>[6x]MADFKFEPMRSLIYVDCVSEDYRPKLQRWIYKVHIPDSISQFEPYVTKYAFYPSFPIPPQGDRFGYARMQLTEHHWLVSDLDPRLEIKAIAETFPMDVLVWQGQIPAAAHTDAQIDSDGDAGNAARKSNNAEGNPFIFAFLPMWWEKDLKGKGRTIEDGANYRFNMTIGFPEGVDKAEGEKWLFEKVVPILQAAPECTRVLASAVKKDING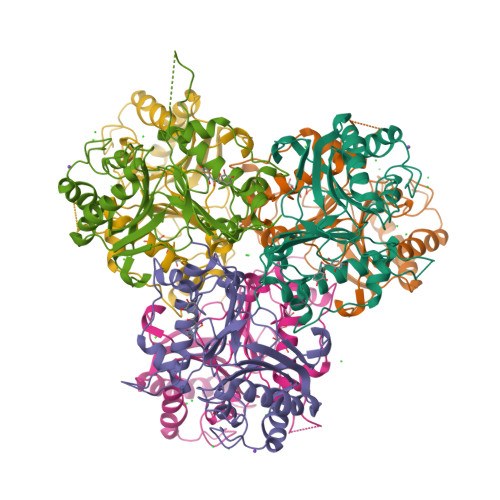CVMDWVLEIWFENQSGWYKVMVDDMKALEKPSWAQQDAFPFLKPYHNVCSAAVADYTPSNNLANYRGYITMR1-pyridin-4-ylthiourea 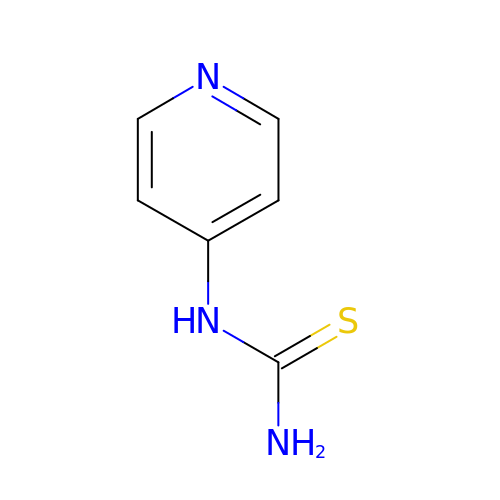| C6 H7 N3 S | HLOFIQOOOSRNFY-UHFFFAOYSA-N>GKAFDDGAFTGIREINLSYNKETAIGDFQVVYDLNGSPYVGENHKSFITGFTPVKISLDFPSEYIMEVSGYTGKVSGYVVVRSLTFKTNKKTYGPYGVTSGTPFSLPIENGLIVGFKGSIGYWLDYFSMYLSL[4x];>[4x]NEQSGISQTVIVGPWGAQV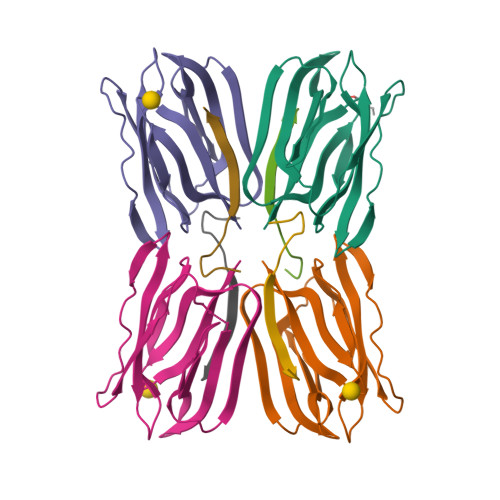ST> MFENITAAPADPILGLADLFRADERPGKINLGIGVYKDETGKTPVLTSVKKAEQYLLENETTKNYLGIDGIPEFGRCTQELLFGKGSALINDKRARTAQTPGGTGALRVAADFLAKNTSVKRVWVSNPSWPNHKSVFNSAGLEVREYAYYDAENHTLDFDALINSLNEAQAGDVVLFHGCCHNPTGIDPTLEQWQTLAQLSVEKGWLPLFA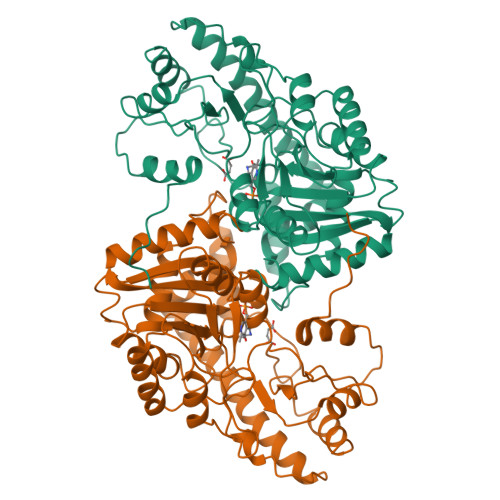FAYQGFARGLEEDAEGLRAFAAMHKELIVASSYSKNFGLYNERVGACTLVAADSETVDRAFSQMKAAIRANYSNPPAHGASVVATILSNDALRAIWEQELTDMRQRIQRMRQLFVNTLQEKGANRDFSFIIKQNGMFSFSGLTKEQVLRLREEFGVYAVASGRVNVAGMTPDNMAPLCEAIVAVL> GPHMGNIMSASFAPECTDLKTKYDSCFNEWYSEKFLKGKSVENECSKQWYAYTTCVNAALVKQGIKPALDEAREEAPFENGGKL

Recently, Ups1, a yeast member of the conserved mitochondrial intermembrane space (IMS) proteins, was shown to mediate PA transfer between the mitochondrial OM and IM in cooperation with Mdm35. Mdm35, another conserved yeast IMS protein, is a binding partner of Ups proteins, and facilitate their import into mitochondria. Surprisingly, two distinct polypeptides of Ups1 and Mdm35 form a single compact domain, the Ups1 part of which corresponds to the START (StAR-related lipid-transfer) domain, likely functioning as a lipid-binding domain. Like other START domain-containing proteins, the Ups1–Mdm35 complex contains a deep pocket that can accommodate a lipid molecule and an Ω-loop likely functioning as a lid for the pocket.

Although full-length Mdm35 (86 residues) failed to crystallize, Mdm35ΔC5 lacking the C-terminal five residues grew crystals suitable for structural analyses. The crystal structure of Mdm35ΔC5 was thus determined from its seleno-methionine (SeMet)-labelled protein crystal by the multiwavelength anomalous dispersion method using the anomalous signal of selenium atoms and was subsequently refined to 1.45-Å resolution against the data set from the native crystal. Residues 67–81 did not exhibit defined electron density, suggesting that the C-terminal segment is disordered in solution. Mdm35 possesses a twin CX9C motif, which is indicative of the substrate for the Tim40/MIA import pathway. Mdm35 contains a short α-helix (α0) and two long α-helices (α1 and α2), which form an antiparallel α-hairpin that is covalently paired by two disulfide bridges, Cys13–Cys52 and Cys23–Cys42.While chemical methylation of an amide bond uses a strong base to generate the imidate, OphA, the precursor protein of the fungal peptide macrocycle omphalotin A, self-hypermethylates amides at pH 7 using S-adenosyl methionine (SAM) as cofactor. Omphalotin A derives from the C terminus of the OphA protein, and it is the OphA protein that methylates its own C terminus using S-adenosyl methionine (SAM). The structure of OphA reveals a complex catenane-like arrangement in which the peptide substrate is clamped with its amide nitrogen aligned for nucleophilic attack on the methyl group of SAM. Here, we report the structure of the peptide amide methyltransferase OphA including complexes with cofactor [SAM and S-adenosyl homocysteine (SAH)], cofactor analog, substrate, and product.

Y76F and Y98A led to highly aggregated protein, and only a small amount could be purified for analysis; very little folded material was obtained for Y98F, but no methylation was detected. Y76F, R72A, R72K, and Y98A were unmethylated even after 3 days of overexpression in E. coli. During prolonged (12 days) incubation, there was some evidence for a very small amount of methylation in the Y98A mutant (>100-fold reduced in vitro activity), but not in the Y76F mutant. A different conformation of Tyr98 is seen in inactive mutant complexes (Y76F-SAM, Y76F-SAH, and R72A-SAH). Y66F retains activity, and Tyr76, although within 4 Å of the carbonyl, has a Bürgi-Dunitz (44°) angle incompatible with attack, so both possibilities were discarded. Both Tyr66 and Tyr76 are, however, well positioned to stabilize the resulting tetrahedral carbon by hydrogen bonding. We therefore hypothesize that, by disrupting anchoring interactions, the flipped conformation can be adopted to relieve the steric clashes between SAM and the amide that would otherwise occur. We speculate that the flipped conformation of the substrate (seen in R72A, Y98A, and Y76F SAM complex structures) resembles an intermediate arrangement that occurs during translocation.

>GTSTQTKAGSLTIVGTGIESIGQMTLQALSYIEAAAKVFYCVIDPATEAFILTKNKNCVDLYQYYDNGKSRLNTFTQMSELMVREVRKGLDVVGVFYGHPGVFVNPSHRALAIAKSEGYRARMLPGVSAEDCLFADLCIDPSNPGCLTYEASDFLIRDRPVSIHSHLVLFQVGCVGIADFNFTGFDNNKFGVLVDRLEQEYGAEHPVVHYIAAMMPHQDPVTDKYTVAQLREPEIAKRVGGVSTFYIPPKARKASNLDIIRRLELLPAGQVPDKKARIYPANQWEPDVPEVEPYRPSDQAAIAQLADHAPPEQYQPLATSKAMSDVMTKLALDPKALADYKADHRAFAQSVPDLTPQERAALELGDSWAIRCAMKNMPSSLLDAARESGEEASQNGFPWVIVVGVIGVIG[2x]> SGDRSMVEVLADHPGELVRTDSPNFLSSVLPTHW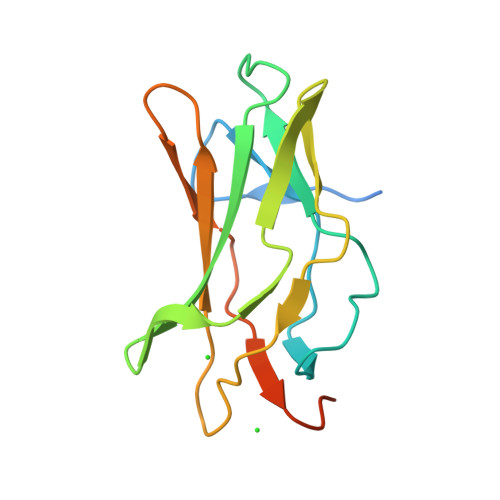RSNKTLPIAFKVVALGDVPDGTLVTVMAGNDENYSAELRNATAAMKNQVARFNDLRFVGRSGRGKSFTLTITVFTNPPQVATYHRAIKITVDGPREPRRHRQKLDD> MGTLTNPFYPIFYYEDFGAVNQGYSVQIVKNTNSQNEAQIGKRVNDIPDAADSNNEFTEARPANRIPANSARNQKAIAIVGTSSNTNYELEAWVTMPIIDVSKNNQYINADDTFKYVSFWTEQRYANGGISSLEVFISTDYTNNV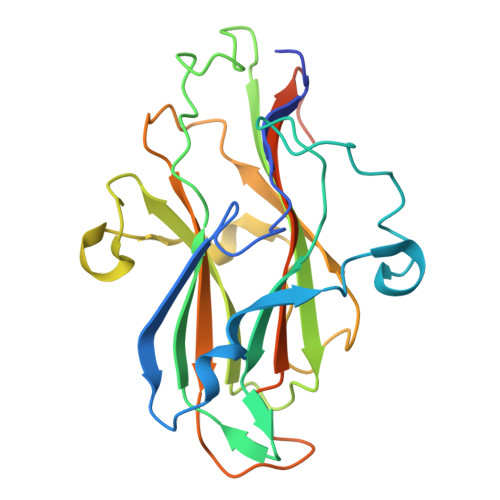TTANWTNVTSNVNKIATSGQNPQTYVESLLDISSYTDTNFTLAFKYTSDNSTYSGSNRNGTFYISDVKYFVSDTTLSNTSFIIEDTIKLEHHHHHH> MHHHHHHSRYEHIPGPPRPSFLLGHLPCFWKKDEVGGRVLQDVFLDWAKKYGPVVRVNVFHKTSVIVTSPESVKKFLMSTKYNKDSKMYRALQTVFGERLFGQGLVSECNYERWHKQRRVIDLAFSRSSLVSLMETFNEKAEQLVEILEAKADGQTPV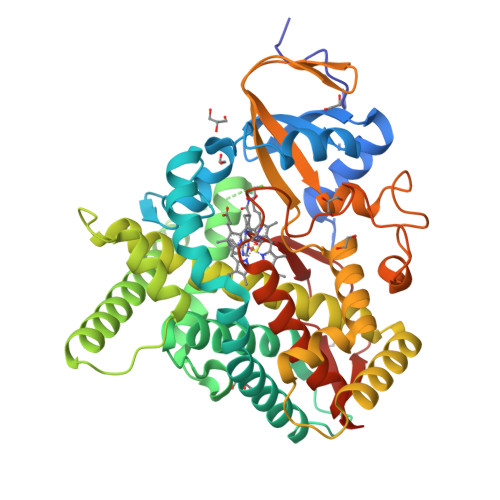SMQDMLTYTAMDILAKAAFGMETSMLLGAQKPLSQAVKLMLEGITASRNTLAKFLPGKRKQLREVRESIRFLRQVGRDWVQRRREALKRGEEVPADILTQILKAEEGAQDDEGLLDNFVTFFIAGHETSANHLAFTVMELSRQPEIVARLQAEVDEVIGSKRYLDFEDLGRLQYLSQVLKESLRLYPPAWGTFRLLEEETLIDGVRVPGNTPLLFSTYVMGRMDTYFEDPLTFNPDRFGPGAPKPRFTYFPFSLGHRSCIGQQFAQMEVKVVMAKLLQRLEFRLVPGQRFGLQEQATLKPLDPVLCTLRPRGWQPA>[2x]MKLSGGVEWALHCCVVLTAASRPVPAARLAELHDVSPSYLAKQMQALSRAGL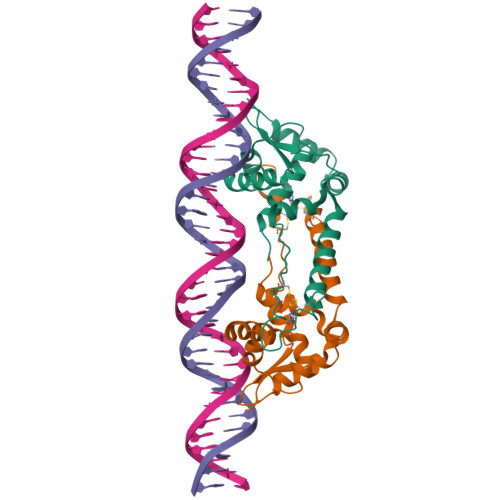VRSVQGKTGGYVLTRPAVEITLLDVVQAVDGPDPAFVCTEIRQRGPLATPPEKCTKACPIARAMGAAEAAWRASLAATTIADLVATVDDESGPDALPGVGAWLIEGLGHHHHHH5-amino-N-[(2S)-2-({[(2,6-dichlorophenyl)carbonyl](ethyl)amino}methyl)-3,3,3-trifluoro-2-hydroxypropyl]-1-(4-fluorophenyl)-1H-pyrazole-4-carboxamide | C23 H21 Cl2 F4 N5 O3 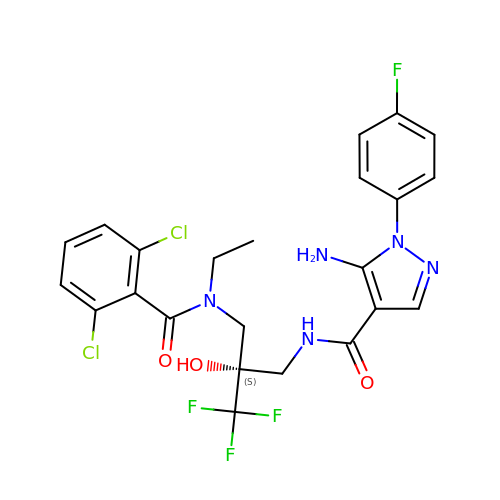| LKQMULLPLYLIGW-QFIPXVFZSA-N>[5x]MALSKVKLNDTLNKDQLLSSSKYTIQRSTGDSIDTPNYDVQKHINKLCGMLLITEDANHK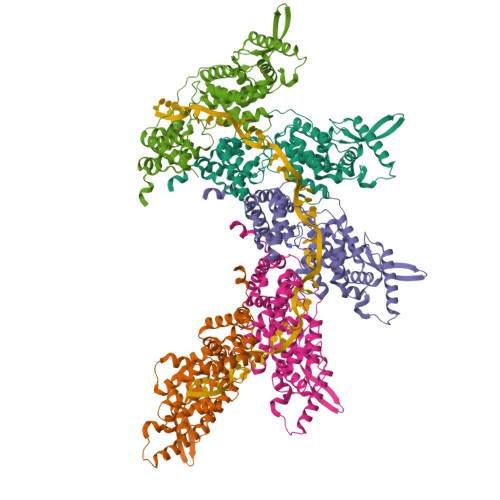FTGLIGMLYAMSRLGREDTIKILRDAGYHVKANGVDVTTHRQDINGKEMKFEVLTLASLTTEIQINIEIESRKSYKKMLKEMGEVAPEYRHDSPDCGMIILCIAALVITKLAAGDRSGLTAVIRRANNVLKNEMKRYKGLLPKDIANSFYEVFEKHPHFIDVFVHFGIAQSSTRGGSRVEGIFAGLFMNAYGAGQVMLRWGVLAKSVKNIMLGHASVQAEMEQVVEVYEYAQKLGGEAGFYHILNNPKASLLSLTQFPHFSSVVLGNAAGLGIMGEYRGTPRNQDLYDAAKAYAEQLKENGV>[2x]MGSLPTNNLESISLCSQNPLDPDEFRRQGHMIIDFLADYYKNVEKYPVRSQVEPGYLKKRLPESAPYNPESIETILEDVTNDIIPGLTHWQSPNYFAYFPSSGSIAGFLGEMLSTGFNVVGFNWMSSPAATELESIVMNWLGQMLTLPKSFLFSSDGSSGGGGVLQGTTCEAILCTLTAARDKMLNKIGRENINKLVVYASDQTHCALQKAAQIAGINPKNVRAIKTSKATNFGLSPNSLQSAILADIESGLVPLFLCATVGTTSSTAVDPIGPLCAVAKLYGIWVHIDAAYAGSACICPEFRHFIDGVEDADSFSLNAHKWFFTTLDCCCLW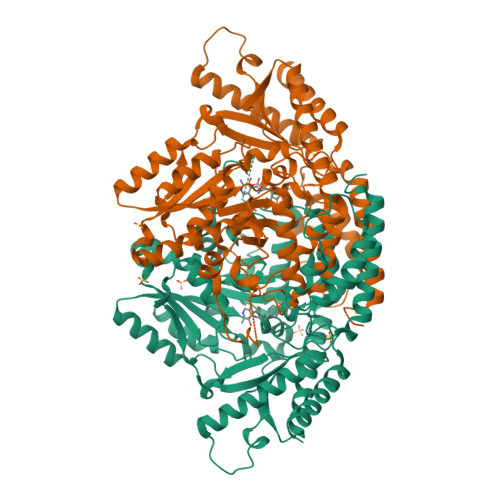VKDSDSLVKALSTSPEYLKNKATESKQVIDYKDWQIALSRRFRSMKLWLVLRSYGVANLRTFLRSHVKMAKHFQGLIGMDNRFEIVVPRTFAMVCFRLKPTAIFKQKIVDNDYIEDQTNEVNVKLLESVNASGKIYMTHAVVGGVYMIRFAVGATLTEERHVTGAWKVVQEHTDAILGA> MDVIKK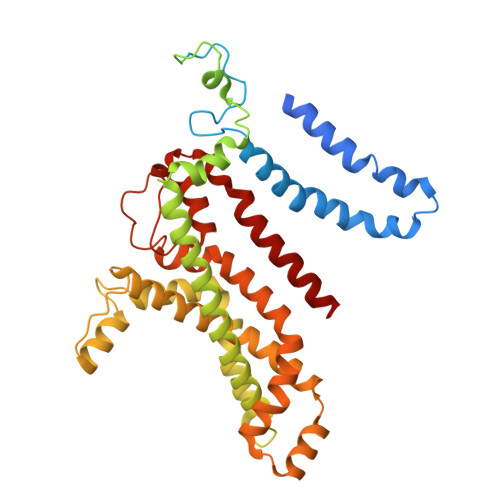KHWWQSDALKWSVLGLLGLLVGYLVVLMYAQGEYLFAITTLILSSAGLYIFANRKAYAWRYVYPGMAGMGLFVLFPLVCTIAIAFTNYSSTNQLTFERAQEVLLDRSWQAGKTYNFGLYPAGDEWQLALSDGETGKNYLSDAFKFGGEQKLQLKETTAQPEGERANLRVITQNRQALSDITAILPDGNKVMMSSLRQFSGTQPLYTLDGDGTLTNNQSGVKYRPNNQIGFYQSITADGNWGDEKLSPGYTVTTGWKNFTRVFTDEGIQKPFLAIFVWTVVFSLITVFLTVAVGMVLACLVQWEALRGKAVYRVLLILPYAVPSFISILIFKGLFNQSFGEINMMLSALFGVKPAWFSDPTTARTMLIIVNTWLGYPYMMILCMGLLKAIPDDLYEASAMDGAGPFQNFFKITLPLLIKPLTPLMIASFAFNFNNFVLIQLLTNGGPDRLGTTTPAGYTDLLVNYTYRIAFEGGGGQDFGLAAAIATLIFLLVGALAIVNLKATRMKFD> MITIVVIPTAHFSWTDTNFLNSVDYRLTSQPKIRDRFAVYAPGWLRRQLDEFSASLTASELLQALQTIPIPVKARCLLLPKPKRFAQWLLDVPSANIWHIPVTTLRATVASKHPSSDVYNYIPDHVPPNAEFDTVTRRVAAGRDIYVRSTKVIGAPLCLAAPAKYYAGYLSTHQLDGIYPENWAPDNFHKREFCLTILPSLLGPRTFLLDVDADRDASYPLSVLWPQLRALALKSRLLLPPVALLRRVVDPGLKPTWSADSDAAFRALRLSRPSSASKPVGFDFSALPVVDIICLLESEPDDHGRIAPGTRLTIHSVPTDLLTSLSIQEGVRYPLRQESGMFVHWVLLALLMSDDVTISGTRRSVKLETAHASARPFVHITVERCASARIIDVRGSPAMYANAVCLTLPKGSYKSTIIDTLPAMFSDLPILEQAAVIDSDALGDSLRPSFETQFLERLENLDPNLLDRAVASILSPTSDTSDDAVTTVLDAFNALYREIMTPAQRARLPLLTQQGRVLAFAHSDYELLSANIPIQVVRGSIPIDHVVNLLARRNRVGGTALQVLLDYCYRTQASPLAPTPAGRLYKQLFGPWLMVPRLSEPLIKLRLVASAPAKVLRAAGWTIDGDPPLEVSCLCAYVTDRAAATALIERRLDSRALVTVGGDQLMFVEYAPPLPLVSIPRTFLLP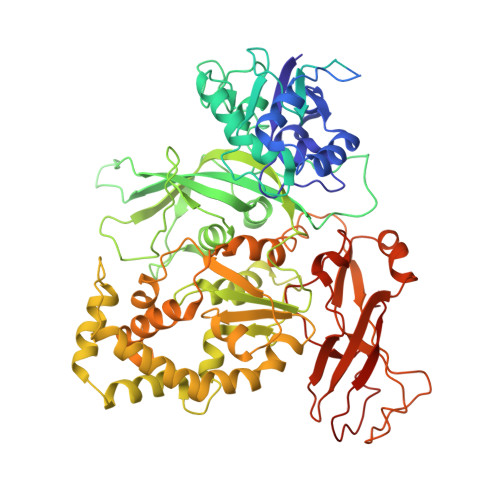VTYVVHWVPPQRVLLNGGNVSFTSGLEWTFDDDPQVVTSTGV STREPTOLYDIGIN | 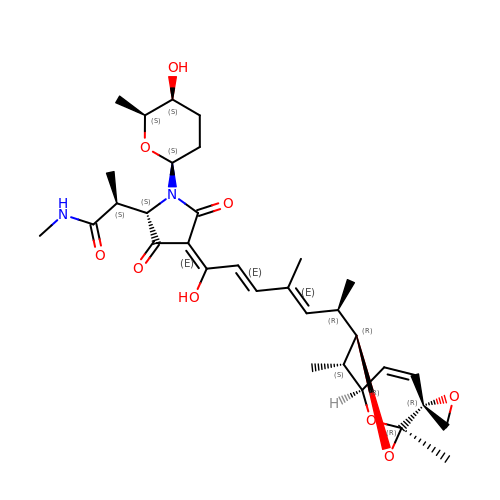C32 H44 N2 O9 | KVTPRMVXYZKLIG-NCAOFHFGSA-N> SSWFLQATNKQMSLTPLFEELLLRCPPKIKSNKGHMASAYQLAQGNWEPLDCGVHLGTIPARRVKIHPYEAYLKLKDLLEEEEKKPKCRDTVIREHNKWILKKVRHQGNLNTKKTLNPGKLSEQLDREGHKRNIYNNQIGTIMTEAGIRLEKLPVVRAQTDTKSFHEAIRDKIDKNENQQSPGLHDKLLEIFHTIAQPSLRHTYSDVTWEQLEAGVNRKGAAGFLEKKNVGEVLDSEKHLVEQLIRDLKTGRKIR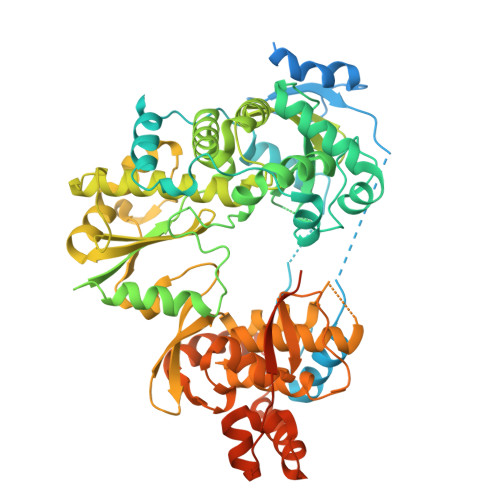YYETAIPKNEKRDVSDDWQSGDLVDEKKPRVIQYPEAKTRLAITKVMYNWVKQQPVVIPGYEGKTPLFNIFNKVRKEWDLFNEPVAVSFDTKNWDTQVTSRDLRLIGEIQKYYYRKEWHKFIDTITDHMVEVPVITADGEVYIRNGQRGSGQPDTSAGNSMLNVLTMMYAFCESTGVPYKSFNNRVARIHVCGDDGFLITEKGLGLKFANNGMQILHEAGKPQKITEGERMKVAYRFEDIEFCSHTPVPVRWSDNTSSYMAGRDTAVILSKMATRLDSSGERGTIAYEKAVAFSFLLMYSWNPLVRRICLLVLSQQPETTPSTQTTYYYKGDPIGAYKDVIGKNLCELKRTGFEKLANLNLSLSTLGIWSKHTSKRIIQDCVTIGKEEGNWLVNADRLISSKTGHLYIPDKGYTLQGKHYEQLQLQARTSPVTGVGTERYKLGPIVNLLLRRLRVLLMAAVGASS> PDHTFTIYYYNE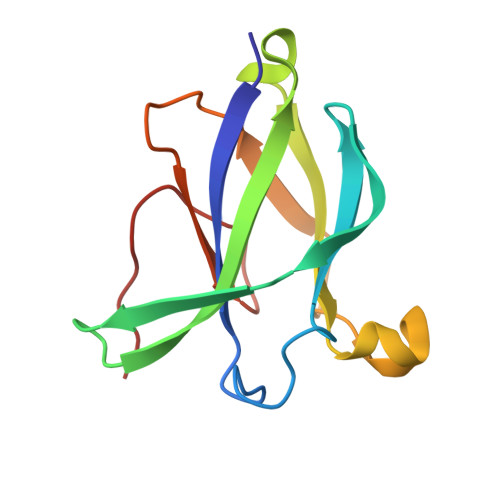DLSTDTDMGKVDLWMWNAGLDGSYVFDGTYYDAENKVTWFKQTITVAGSNVGKTVGLKARYDNTKGWDGGSDTADRSFTISGDENEVLYYVDGSDPVHEKPVIV1-[2-(4-ETHOXY-3-FLUOROPYRIDIN-2-YL)ETHYL]-3-(5-METHYLPYRIDIN-2-YL)THIOUREA 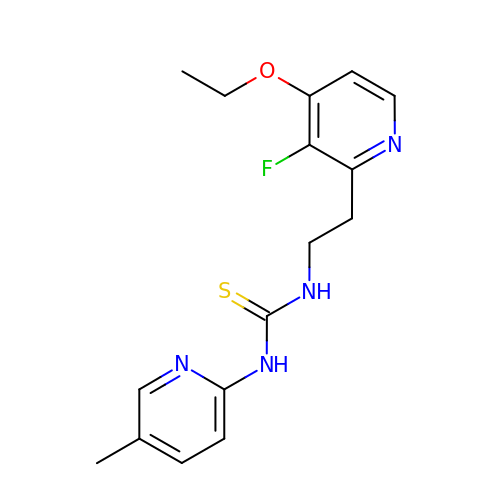| C16 H19 F N4 O S | QOVMZMFNTIUFLU-UHFFFAOYSA-N>GAMLSTLPVPPSQRDNLEASFAIVSAEECDPTDDICEIGVRMEEQ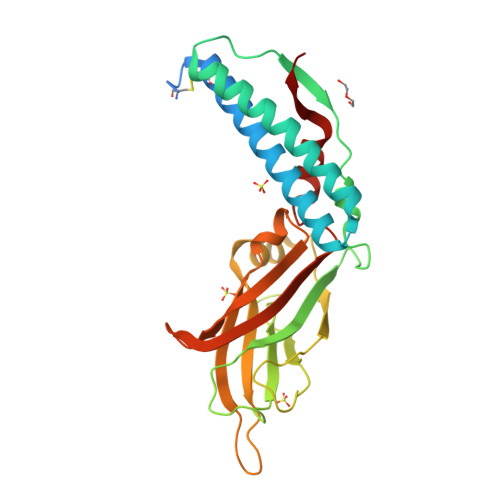LAKQLMMCKNTRDHHKAMGDVAGMNRFENLALTVQKDLDLVRYSKRKNEPLPKFHYEKRSFNIVHCNTDLTDSELEIVVVRGISYNVANPKDVDTYVRVEFPLLNDESFKTKTNVIRDTSSPDYDERFKVDIQRTNRQFQRIFKRHGVKFEIYSRGGFLRSDTLIGTVNVKLQPLETKCEIHDTYDLMDGRKQVGGKLEVKIRVRNPILTKQMEHITEKWLVLDA[2x]> GSMSTINFANREINFKIVYYGPGLSGKTTNLKWIYSKVPEGRKGEMVSLATEDERTLFFDFLPLDIGEVKGFKTRFHLYTVPGQVFYNASRKLILRGVDGIVFVADSAPNRLRANAESMRNMRENLAEYGLTLDDVPIVIQVNKRDLPDALPVEMVRAVVDPEGKF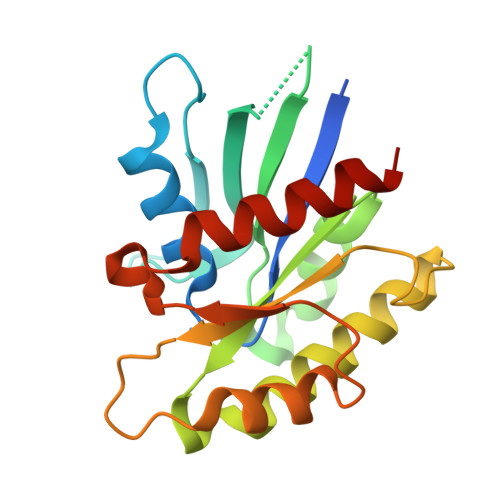PVLEAVATEGKGVFETLKEVSRLVLARVAGGS>[4x]AAMEQFRQIGEVLGSLNALMVLQDDILINQRQCCLLLELFSLAFNTVAEEIRQNLKLEEKHTKWRALEQPLRELTRVFKEGELYVKHCMDNSDWWGKVINLHQNKDCVEFHIHNLFCYFSAVVEAIEAAGEISGLDPSEMERRRVVFSRKYDREWNDPKMFQWRFGKQYLLSRDICSRFEHSWREDRWNLVEALQEKRKSDSDDIGKTEKRLADLLLKKLTGLEQFNGKLFPSSILLGSKDYQVKKRLDADGQYKEIQWLGDSFALRHFFSDLEPLSSEISSLLALCHSNILQYLCGFYDEERKECFLVMELMHKDLQSYMKENCGPRRRYLFSIPVVIDIMLQIARGMEYLHGNDIFHGDLNP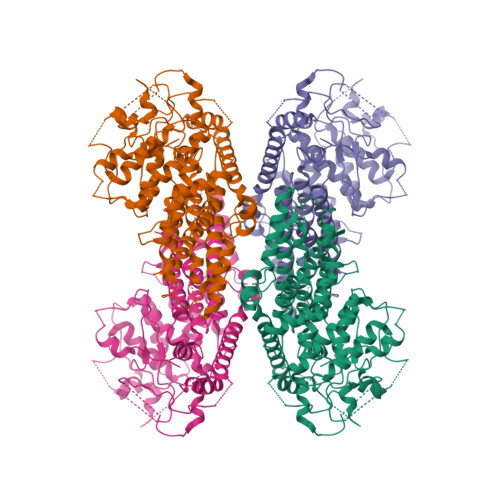MNIHLKERSHTEGYFHAKICGFGLSSVVKAQSSSKPGTPDPVIWYAPEVLAEMEQDLNGKTPKSKLTHKADVYSFAMVCFELITGKVPFEDSHLQGEPMTINIRMGERPLFPFPSPKTLVSLIKRCWHSEPSQRPNFSSICRILRYIKKFLVVNPDHGHPQMQTPLVDCWDLEARFLRKFPGDAGSHTASVNQIPFQLTSYRVLEKEK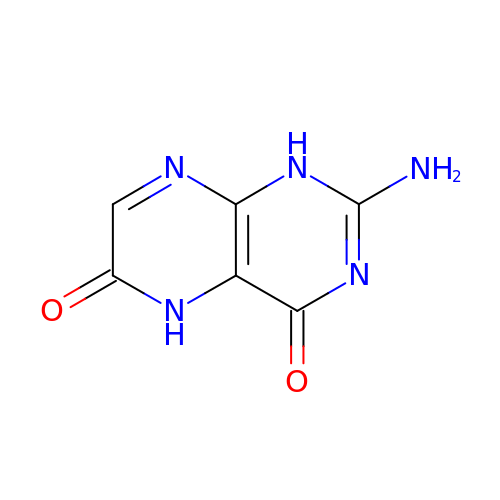2-amino-1,5-dihydropteridine-4,6-dione | C6 H5 N5 O2 | VURKRJGMSKJIQX-UHFFFAOYSA-N> GAGCAGACGTGA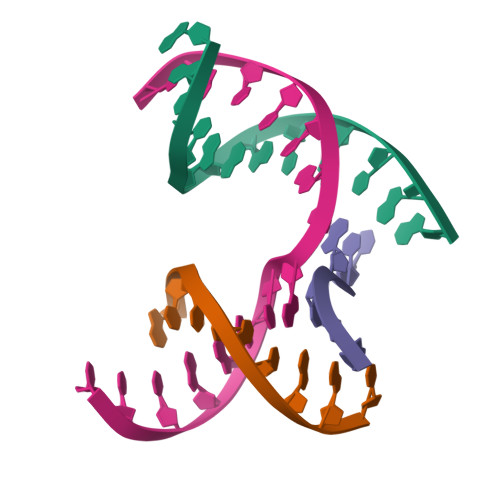;> CGACACTCA;> TCATCG;> TCTGAGTGCGTCTGC> GASQFFKDNCNRTTASLVEGVELTKYISDINNNTDGMYVVSSTGGVWRISRAKDYPDNVMTAEMRKIAMAAVLSGMRVNMCASPASSPNVIWAIELEAE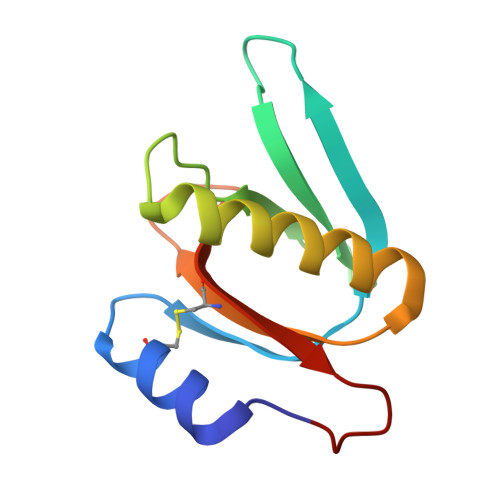GSGS> MEKSFVITDPRLPDNPIIFASDGFLELTEYSREEILGRNGRFLQGPETDQATVQKIRDAIRDQREI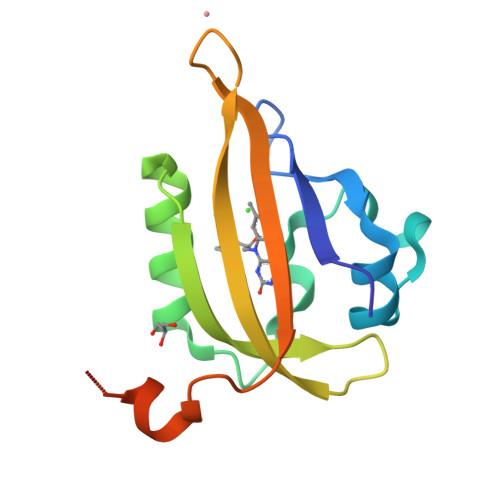TVQLINYTKSGKKFWNLLHLQPMRDQKGELQYFIGVQLDGEFIPNPLLGLDSTRTGHHHHHHD>[2x]MQAKIKNKRVLVKFSGEALAGDNQFGIDIHV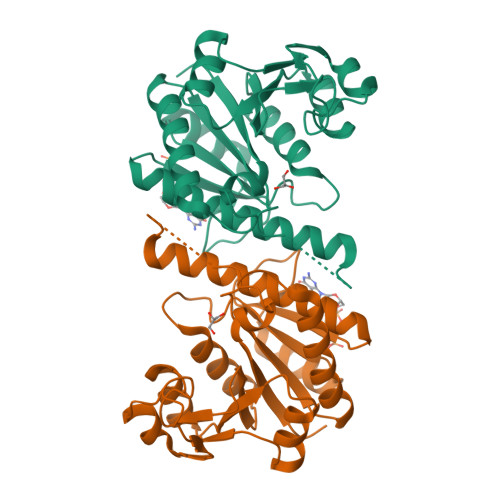LDHIAKEIKSLVENDIEVGIVIGGGNIIRGVSAAQGGIIRRTSGDYMGMLATVINAVAMQEALEHIGLDTRVQSAIEIKEICESYIYRKAIRHLEKGRVVIFGAGTGNPFFTTDTAATLRAIEIGSDLIIKATKVDGIYDKDPNKFKDAKKLDTLSYNDALIGDIEVMDDTAISLAKDNKLPIVVCNMFKKGNLLQVIKHQQGVFSMVK> MAHHHHHHVGTGSNDDDDKSPDPWELTILHTNDVHSRLEQTSEDSSKCVDASRCMGGVARLFTKVQQIRRAEPNVLLLDAGDQYQGTIWFTVYKGAEVAHFMNALRYDAMALGNHEFDNGVEGLIEPLLKEAKFPILSANIKAKGPLASQISGLYLPYKVLPVGDEVVGIVGYTSKETPFLSNPGTNLVFEDEITALQPEVDKLKTLNVNKIIALGHSGFEMDKLIAQKVRGVDVVVGGHSNTFLYTGNPPSKEVPAGKYPFIVTSDDGRKVPVVQAYAFGKYLGYLKIEFDERGNVISSHGNPILLDSSIPEDPSIKADINKWRIKLDDYSTQELGKTIVYLDGSSQSCRFRECNMGNLICDAMINNNLRHADEMFWNH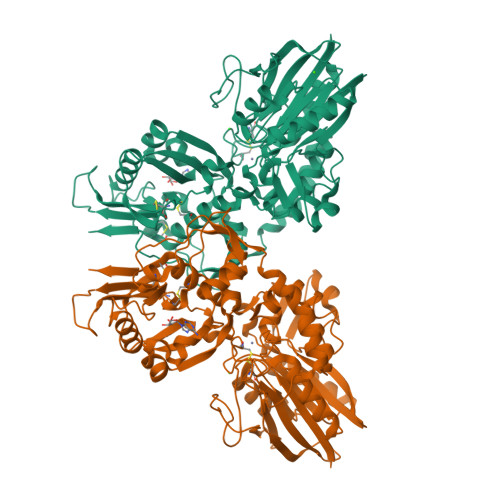VSMCILNGGGIRSPIDERNDGTITWENLAAVLPFGGTFDLVQLKGSTLKKAFEHSVHRYGQSTGEFLQVGGIHVVYDLSRKPGDRVVKLDVLCTACAVPSYDPLKMDEVYKVILPNFLANGGDGFQMIKDELLRHDSGDQDINVVSTYISKMKVIYPAVEGRIKFS>ETHTFNWTTGWDYRNVDGLKSRPVITCNGQFPWPDITVNKGDRVQIYLTNGMNNTNTSMHFHGLFQNGTASMDGVPFLTQCPIAPGSTMLYNFTVDYNVGTYWYHSHTDGQYEDGMKGLFIIKDDSFPYDYDEELSLSLSEWYHDLVTDLTKSFMSVYNPTGAEPIPQNLIVNNTMNLTWEVQPDTTYLLRIVNVGGFVSQYFWIEDHEMTVVEIDGITTEKNVTDMLYITVAQRYTVLVHTKNDTDKNFAIMQKFDDTMLDVIPSDLQLNATSYMVYNKTAALPTQNYVDSIDNFLDDFYLQPYEKEAIYGEPDHVITVDVVMDNLKNGVNYAFFNNITYTAPKVPTLMTVLSSGDQANNSEIYGSNTHTFILEKDEIVEIVLNN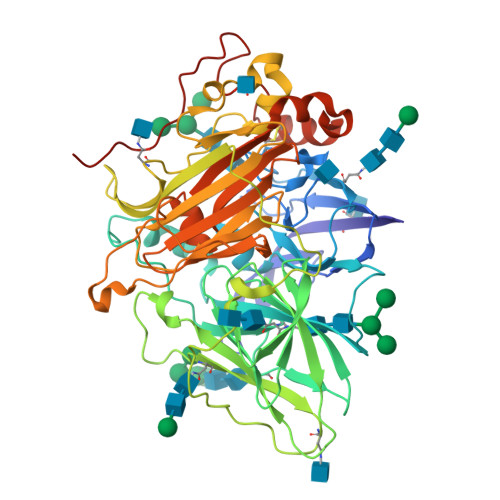QDTGTHPFHLHGHAFQTIQRDRTYDDALGEVPHSFDPDNHPAFPEYPMRRDTLYVRPQSNFVIRFKADNPGVWFFHCHIEWHLLQGLGLVLVEDPFGIQDAHSQQLSENHLEVCQSCSVATEGNAAANTLDLTDLTGENVQHAFIPTG[6x]(2E,6E)-7,11-dimethyldodeca-2,6,10-trien-1-yl trihydrogen diphosphate 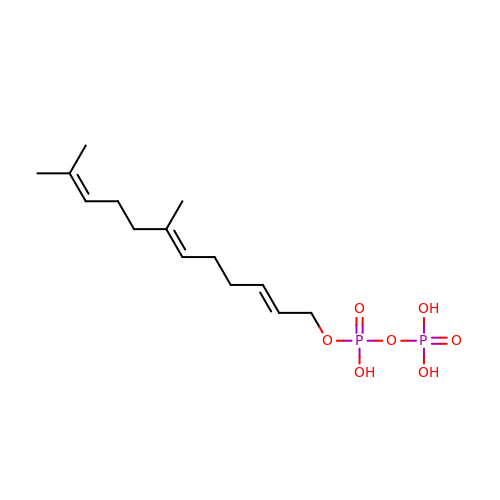| C14 H26 O7 P2 | AFSHNJXUHHFZPQ-XOBXVUKQSA-N Here, we provide the ligand/enzyme crystal complexes for one such PTP outlier: Arabidopsis thaliana Plant and Fungi Atypical Dual Specificity Phosphatase 1 (AtPFA-DSP1), herein unveiled as a regioselective and efficient phosphatase towards inositol pyrophosphate (PP-InsP) signaling molecules. Although the WPD loop is missing its canonical tripeptide motif, this structural element contributes to catalysis by assisting PP-InsP delivery into the catalytic pocket, for a choreographed exchange with phosphate reaction product. Subsequently, an intramolecular proton donation by PP-InsP substrate is posited to substitute functionally for the absent aspartate/glutamate general-acid. Additionally, we conclude that the hydrolyzed phosphate remains trapped as an enzyme-product complex, until it can be released in a prisoner exchange with another PP-InsP molecule; the latter process is assisted by the WPD loop.

The oxygen atom that is positioned at the apex of the phosphate ion’s tetrahedral geometry points away from α4. This oxygen makes a hydrogen bond with the unprotonated Nδ1 of His155 (we will return to this point below). We denote this orientation of Pi as pose A, i.e., Pi(A). The three other oxygen atoms of this Pi are intensively coordinated by amide groups of P-loop residues Lys151, Arg152 Lys154, His155, and Arg156. The side chains of Arg156 and Cys150/Ser150 also make polar contacts with Pi(A). Deriving such crystals for AtPFA-DSP1 was initially problematic; we were unable to displace enzyme-associated Pi by soaking crystals of wild type enzyme with 5-InsP7. This observation also speaks to how tightly the enzyme holds on to the Pi product (and see below).

>[2x]GSFTEELHLIPPLNFSMVDNGIFRSGFPDSANFSFLQTLGLRSIIYLCPEPYPESNLQFLKSNGIRLFQFGIEGNKEPFVNIPDHKIRMALKVLLDEKNHPVLIHCKRGKHRTGCLVGCLRKLQKWCLTSIFDEYQRFAAAKARVSDQRFMEIFDVSSFSHIPMSFSCSIR>TRKMWSVQESEWLKQGVVRYGVGHWERIRSAFPFAGRTAV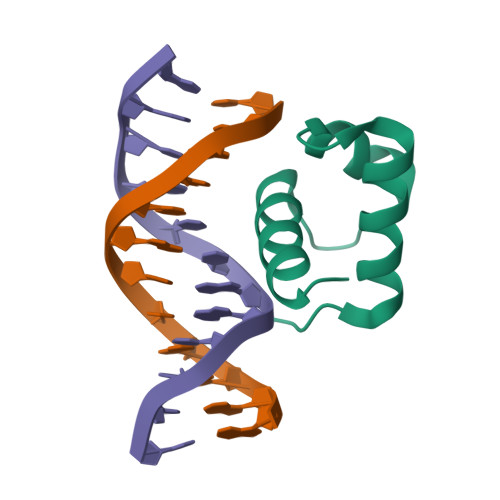NLKDRWRTMVKLKM[2x]> GPLGSMSEEQVAQDTEEVFRSYVFYRHQQEQEAEGVAAPADPEMVTLPLQPSSTMGQVGRQLAIIGDDINRRYDSE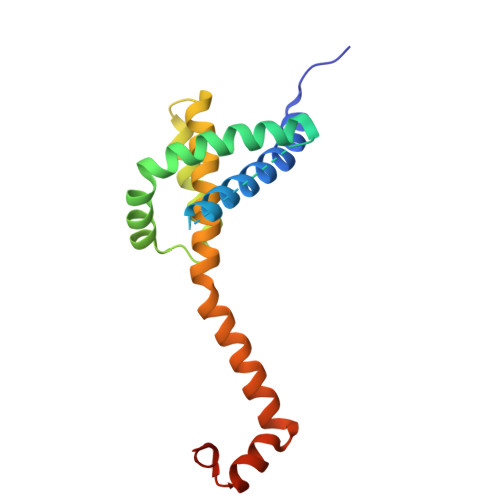FQTMLQHLQPTAENAYEYFTKIATSLFESGINWGRVVALLGFGYRLALHVYQHGLTGFLGQVTRFVVDFMLHHSIARWIAQRGGWVAALNLGNG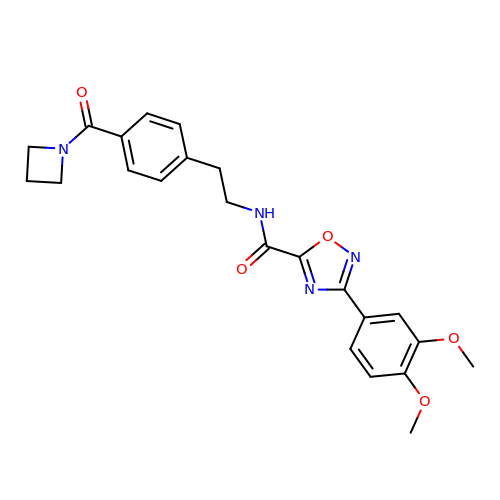~{N}-[2-[4-(azetidin-1-ylcarbonyl)phenyl]ethyl]-3-(3,4-dimethoxyphenyl)-1,2,4-oxadiazole-5-carboxamide | C23 H24 N4 O5 | GCZJCDQGYPXFCY-UHFFFAOYSA-N>HHHHHHSSGLVPRGSHMNAADESLGNVLLVGLGAVAIQVALDLRRHGAGRLGALNHPGRRSQRIAEALARGACLQLEGQGQHRWLSGNAALDVFHQDPAELRDDWQTLVLCVPADSYLDVVRGLPWERLGGVRTLLLVSAFIGANLLVRSALPAGCQATVLSLSSYYAATKVIDETQPLRALTKAVKRRVYLGSSRPDCPARETWRRVLAGSGVEVVPLATPEAAEGRNVTTYVHSPFFLGEFALARILSEQGPPGFMYKLYPEGPITPGAIGAMRRLWCELSELLRRMGAEPLNLLRFLNDDNYPVHETMLPRASIDGFAEAGAERQEYLLFVRYAALLVDPFSPADEQGRHFDFSAVPFRRVSRDEDGLWRLPRVPLEDYRKLALI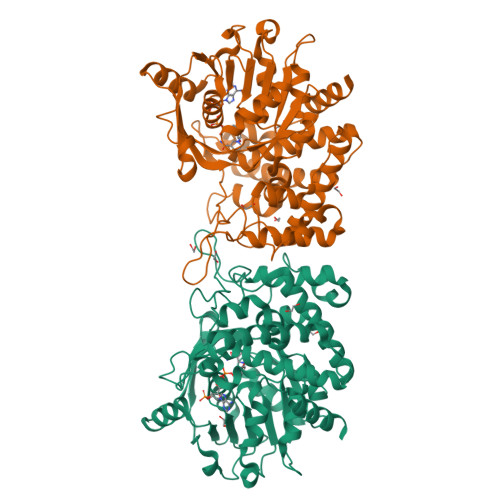VALAAHFDLAMPQARSLLASYENAVSRFIDCQGASQCHPSLYPIDSRPAADAIYRQWCSTC[2x]>[6x]GGEVPIGDPKELNGMEIAAVYLQPIEMEPRGIDLAASLADIHLEADIHALKNNPNGFPEGFWMPYLT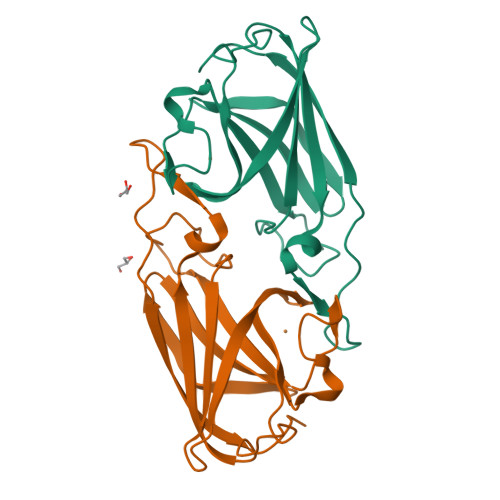IAYELKNTDTGAIKRGTLMPIVADDGPHYGANIAMEKDKKGGFGVGNYELTFYISNPEKQGFGRHVDEETGVGKWFEPFKVDYKFKYTGTPK>[2x]GSFTYTFVVRDENSTVYAEVAKILLASGQWKRLKRDNP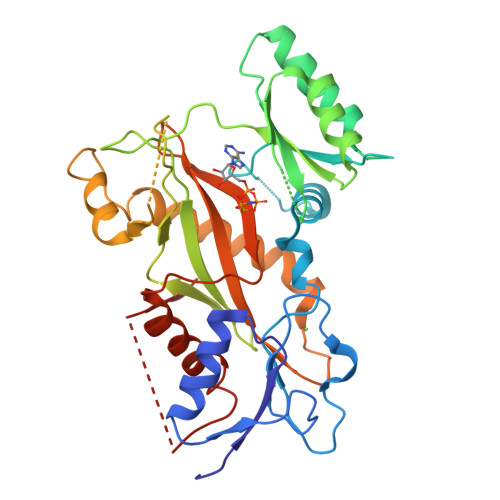KFNLMLGERNRLPFGRLGHEPGLVQLVNYYRGADKLCRKASLVKLIKTSPELTETCTWFPESYVIYPTNEKTPAMRARNGLPDLANAPRTDEREEFRSSFNKKKENEEGNVWIAKSSSGAKGEGILISSDATELLDFIDNQGQVHVIQKYLESPLLLEPGHRKFDIRSWVLVDNQYNIYLYREGVLRTSSEPYSDTNFQDMTSHLTNHCIQKEHSKNYGRYEEGNEMFFEEFNQYLVTSLNINLENSILCQIKEIIRVCLSCLEPAISTKYLPYHSFQLFGFDFMVDKNLKVWLIEVNGAPACAQKLYAELCKGIVDLAISSVFPLNEENHKPTEDNVFIKL2-(5-methoxy-1H-indol-3-yl)ethanamine 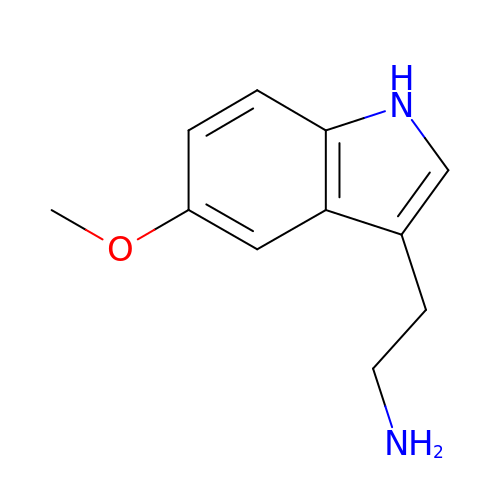| C11 H14 N2 O | JTEJPPKMYBDEMY-UHFFFAOYSA-N Genome segregation is a fundamental process that preserves the genetic integrity of all organisms, but the mechanisms driving genome segregation in archaea remain enigmatic. This study delved into the unknown function of SegC (SSO0033), a novel protein thought to be involved in chromosome segregation in archaea. The segC (sso0033) gene encodes a 165-residue hypothetical protein of unknown function. SegC has a tertiary structure folding similar to those of the ThDP-binding fold superfamily, but SegC shares only 5–15% sequence identity with those proteins. Surprisingly, we found that SSO0033 exhibits nucleotide triphosphatase (NTPase) activity and assembles into filaments in the presence of nucleoside triphosphates (NTPs) and DNA.

To this end, we determined the crystal structure of SegC at 2.8 Å resolution. The monomer structure of SegC exhibits a compact spherical shape consisting of eight α-helices and a five-stranded parallel β-sheet. In addition, the electrostatic surface potential on one side of SegC reveals two positively-charged grooves, which might play a key role in the DNA-binding ability of SegC. In the asymmetric unit, SegC forms a tetramer composed of two types of dimers, i.e. AB and AB'. All four monomers exhibit an almost identical conformation, with the root mean square deviation (r.m.s.d.) ranging from 0.20 to 0.25 Å (in Cα). To determine the most likely interaction interface that could represent a major structural element in tetramer formation, we used the PISA server to measure the surface areas of these two dimer interfaces. The buried surfaces within dimer AB and dimer AB' are 713.4 and 497.4 Å2, respectively (Interface-1 and Interface-2 of Figure 2D, respectively). Therefore, Interface-1 of dimer AB most likely plays a major role in the formation of the SegC dimer, and the interaction between the two dimers contributes to the assembly and stabilization of the entire tetramer. The major residues that contribute to Interface-I are Ile160 and Leu161 from the C-terminal α8 helix of SegC. Furthermore, interactions in the SegC AB' dimer interface (Interface-2) are primarily attributable to loop-rich regions, comprising the α4β2, β2β3 and β3β4 loops of both monomers. We also noticed that two SegC tetramers can assemble into an octamer from two adjacent asymmetric units.

>MFEKLYSAIIYSDEFKKILLGRGVDDLEIASAYIAFLYEDLPIIGKNLCAAFLRMGLDAVYNVMPSGKVYSPRHKLYPISRYGIDGVCINCDGGKIILRISNKGYDPEDLLESKGLESRIFVSKNFKKKSMEIIEKIWDVNKIRLIARKEILERISAGGILHMIRLEHHHHHH[4x]> AQSVPYGVSQIKAPALHSQGYTGSNVKVAVIDSGIDSSHPDLNVAGGASFVPSETNPFQDNNSHGTHVAGTVLAVAPSASLYAVKVLGADGSGQYSWIINGIEWAIANNMDVINMSLGGPSGSAALKAAVDKAVASGVVVVAAAGNEGTSGSSSTVGYPGKYPSVIAVGAVDSSNQRASFSSVGPELDVMAPGVSIVSTLPGNKYGAKSGTAMASPHVAGAAALILSKHPNWTNTQVRSSLENTTTKLGDSFYYGKGL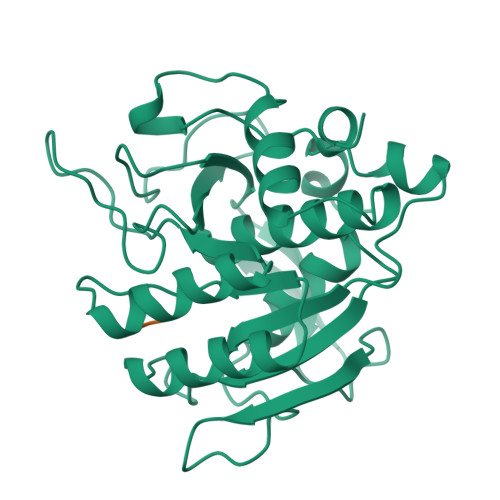INVEAAAQ;> ALAL>[4x]GSHMTNFVLGNAQIVD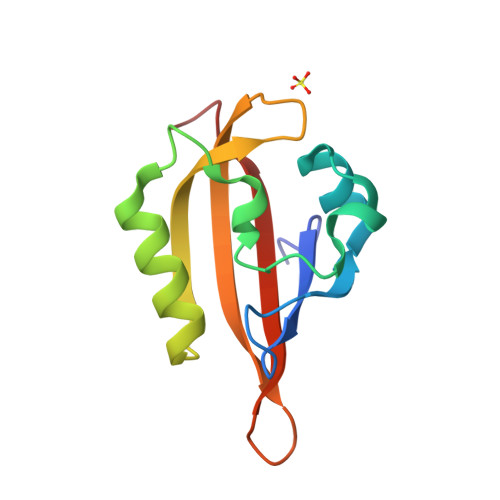WPIVYSNDGFCKLSGYHRAEVMQKSSACSFMYGELTDKDTVEKVRQTFENYEMNSFEILMYKKNRTPVWFFVKIAPIRNEQDKVVLFLCTFSDITAFK> KPKEDREWEKFKTKHITSQSVADFNCNRTMNDPAYTPDGQCKPINTFIHSTTGPVKEICRRATGRVNKSSTQQFTLTTCKNPI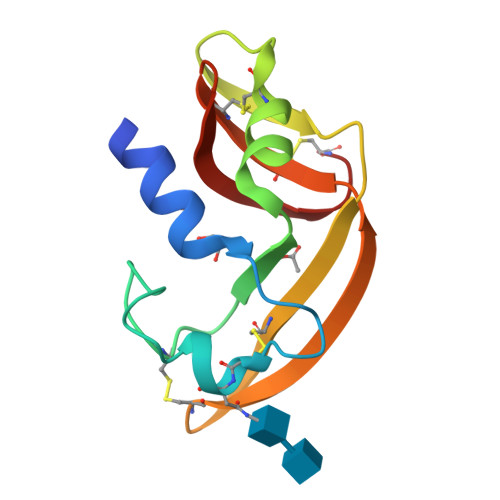RCKYSQSNTTNFICITCRDNYPVHFVKTGKC Here, we elucidated the molecular mechanism underlying the function and regulation of P. fluorescens LapD, a transmembrane receptor essential for biofilm formation in this strain. As c-di-GMP levels change LapD switches between two states: the dinucleotide-unbound off state that retards stable biofilm formation by facilitating the secretion of the cell surface adhesin LapA, and the c-di-GMP-bound on state that supports cell adhesion by preventing the release of LapA from the outer membrane. Binding of c-di-GMP to the LapD EAL domain is relayed to the periplasmic output domain through an inside-out signaling mechanism that utilizes a juxtamembrane HAMP domain, a relay module often found in bacterial transmembrane receptors. Here, we present three crystal structures of LapD from P. fluorescens that provide models for the c-di-GMP-unbound cytoplasmic domain lacking only the HAMP domain, a c-di-GMP-bound EAL domain dimer, and the periplasmic domain.

In order to elucidate the molecular mechanism that regulates LapD function, we determined the crystal structure of the intracellular module of P. fluorescens LapD, comprising a HAMP–GGDEF domain linker segment and the degenerate GGDEF–EAL domain module (LapDdual; residues 220–648). The structure of LapDdual (space group P32, one molecule in the asymmetric unit) was solved by single-wavelength anomalous dispersion phasing using selenomethione-substituted protein crystals. We also obtained a second crystal form involving different crystal packing contacts (space group I23, one molecule in the asymmetric unit), yet the overall structure of LapDdual in the two crystals is identical (root mean square deviation [rmsd] of 0.9 Å over all atoms; Figure S2A and S2C). In both cases, the biologically significant unit was predicted to be a monomer, based on energetic and geometric estimations. LapDdual adopts a compact, bilobal conformation. The GGDEF domain, comprising the N-terminal lobe, caps the dinucleotide-binding pocket of the EAL domain, which forms the C-terminal lobe of the tandem domain structure. The EAL domain buttresses the N-terminal S helix via predominantly hydrophobic interactions, burying 1,170 Å2. In addition to the S helix–EAL domain interaction, the GGDEF domain contacts the dinucleotide-binding surface of the EAL domain at multiple points, forming a loosely packed interface that buries 1,620 Å2 of surface area. One such contact, the salt bridge between an arginine residue (R450) and a glutamate residue (E262), forms a particularly close interaction. While E262 directly occupies the dinucleotide-binding site, the loop itself is located at its periphery, partially blocking access of c-di-GMP to the EAL domain. In summary, the structural analysis of the cytoplasmic domain of LapD reveals that in the absence of c-di-GMP, the protein resides in a conformation incompatible with dinucleotide binding, with the GGDEF domain restricting access of c-di-GMP to the EAL domain.

> AALFQEQAERSEKLRTESYQDNLTGLANRRYFEMQLNARVSNPEQASSGYLLLLRVKDLAGLNQRLGGQRTDELLKAVGEQLSRECAKYPETQNLVTRIRGGEFAVLAPGMTREEALQLAQSLDSALSSLYATGATDVAAVASIGLAPFAHGDSPQAVLSLGDQALAQAEGQGEQNWACLDQSLVADVGDDHHAWHRLLDQALNQRRFELFFQPVVAAQDTQLVLHYKVLSRLLDEQGQTIPAGRFLPWLERFGWTARLDRLMLERVLEQMAGHEESLALNLSSATLADPQALNKVFEILRAHSNLGARLTLEIGEEQLPEQAVLEQLTRRLRELGFSLSLQRFGGRFSMIGNLARLGLAYLKIDGSYIRAIDQESDKRLFIEAIQRAAHSIDLPLIAERVETEGELSVIREMGLYGVQGQLFGEPKPWG1-(2-ethoxyphenyl)-4-[(4-methylphenyl)sulfonyl]-1H-1,2,3-triazol-5-amine 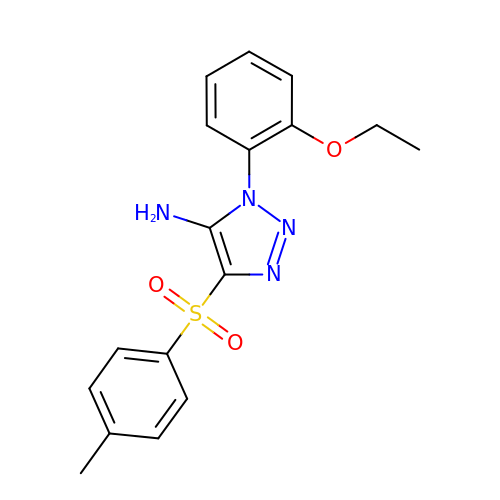| C17 H18 N4 O3 S | IDPPLGOKMUUTFP-UHFFFAOYSA-N>GSMRHPKIPILKLYNCLLVSIQWELDDQTAL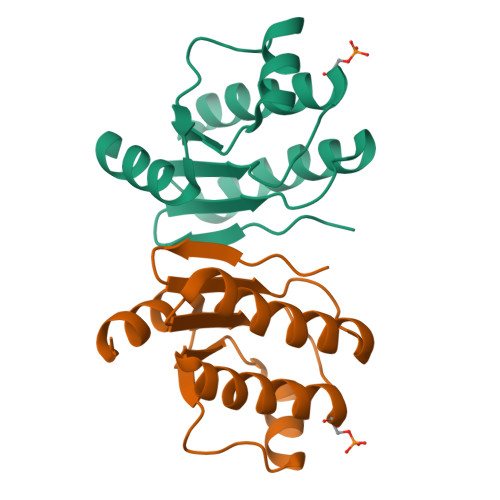TFQEDLLNKIYETGANGVVIDLTSVDMIDSFIAKVLGDVITMSKLMGAKVVLTGIQPAVAVTLIELGIALEEIETALDLEQGLETLKRELGE[5x]>PVDLSKHPSGIVPTLQNIVSTVNLDCKLDLKAIALQARNAEYNPKRFAAVIMRIREPKTTALIFASGKMVCTGAKSEDFSKMAARKYARIVQKLGFPAKFKDFKIQNIVGSCDVKFPIRLEGLAYSHAAFSSYEPELFPGLIYRMKVPKIVLLIFVSGKIVITG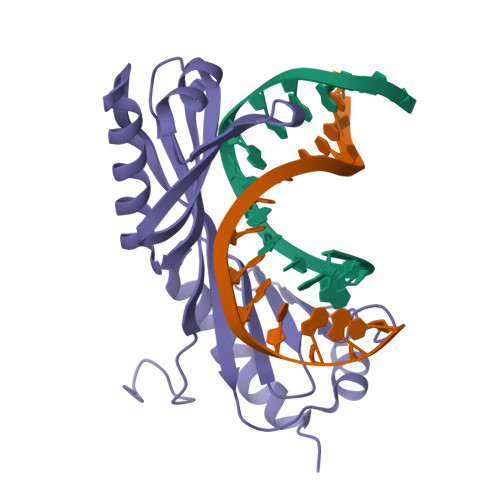AKMRDETYKAFENIYPVLSEFRKIQQ[2x]>GSHMASEKGTVVTETADDDLFTTYRLDLEDARSKEREELNAIVSSDDATAKEKSEAYDKMTALSEVEGTEKQLETLIKTQGYEDALVNAEGDKINITVKSDKHSKSKATAIIDLVAKEIKTMKDVAVTFEPSK[2x];>[2x]GSHMGKSMENVAMPVVDSENVSVVKKFYETDAAKEEKEAALVTYNNTYSLSKGIDLAEKDGKDFDVSASLSGTVVKAEKDPVLGYVVEVEHADGLSTVYQSLSEVSVEQGDKVKQNQVIGKSGKNLYSEDSGNHVHFEIRKDGVA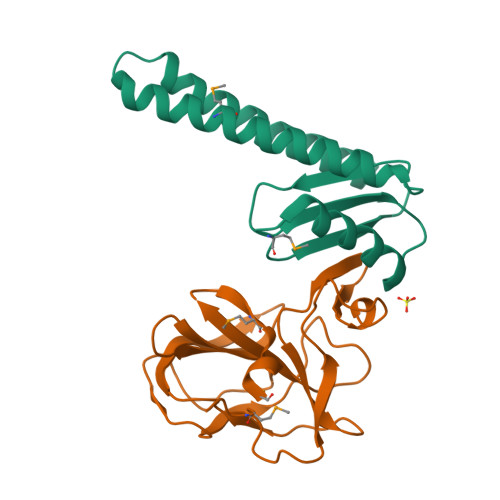MNPLNFM Prokaryotic nanocompartments, also known as encapsulins, are a recently discovered proteinaceous organelle-like compartment in prokaryotes that compartmentalize cargo enzymes. Here, we describe a novel encapsulin in the freshwater cyanobacterium Synechococcus elongatus PCC 7942. This nanocompartment is upregulated upon sulfate starvation and encapsulates a cysteine desulfurase enzyme via an N-terminal targeting sequence. The SrpI encapsulin is 24.5 nm in diameter and has a T = 1 icosahedral capsid formed by the self-assembly of 60 SrpI monomeric subunits, similar to previously reported encapsulin structures.

Holo-SrpI (CyD loaded) was generated by denaturation of the purified SrpI shell protein and re-folding the shell protein in the presence of CyD as described in the previous section. Cryo-EM analysis was performed on purified holo-SrpI to resolve the shell structure at 2.2 Å resolution. This represents the first Family 2 encapsulin structure and is the highest resolution structure for an encapsulin to date, allowing for accurate atomic model building (Figure 6—figure supplements 1 and 2). Interestingly, the A-domain of SrpI that forms a pore at the fivefold axis is composed of residues that are positively charged, in contrast to the negatively charged fivefold axis pore of Family 1 encapsulins. Unfortunately, during processing and classification, the holo-SrpI encapsulin proved nearly indistinguishable from the apo-SrpI control. The inability to resolve significant portions of the cargo density may be due to low occupancy, or conformational flexibility of the cargo, which disappears at higher resolutions when many particles are averaged together. However, symmetry expansion and focused classification of the holo-SrpI encapsulin, guided by the 225-NTD-sfGFP-SrpI dataset, revealed additional EM density at the interior surface of the shell that was localized to the three-fold symmetry axis. While the cargo EM density was too weak to accurately build an atomic model of the cysteine desulfurase cargo residues, we were able to determine which shell residues likely interact with cargo density based on their proximity to the putative cargo EM density. Of note, shell residues at the threefold axis neighboring the cargo EM density are highly conserved, which suggests that the interaction between the encapsulin cargo and shell may be conserved. Namely, residues F262, and Y273 are located near the suggested cargo density.

> MTDNAPQLALRDVAARQLANATKTVPQLRTITPRWLVRLLHWTPVEAGIYRVNQVKDASQITVACSERDESELPETFVDYIDNPREYLLSAVNTVVDVHTRISDLYSNPHDQIREQLRLTIEIMKERQESELINSREYGLLNNVAPGQLVHTRNGAPTPDDLDELLIRVWKEPAFFLAHPQAIAAFGRECTRRGVPPATVSLFGSSFITWRGVPLIPSDKVPLENGKTKILLLRVGESRQGVVGLYQPNLPGEQGMGLSVRFMGINRKALASYLVSLYCSLAVLTDDALAVLDNVDVTQYHTYRYNSGHHHHHH> MHLSLLVPFLFWITGCCTAEDPVTGPEEVSGQEQGSLTVQCRYTSGWKDYKKYWCQGVPQRSCKTLVETDASEQLVKKNRVSIRDNQRDFIFTVTMEDLRMSDAGIYWCGITKGGLDPMFKVTVNIGPVPTMPPITSTTTIFTVTTTVKETSMFPTLTSYYSDNGHGGGDSGGGEDGVGDGFLDLSVLLPVISAVLLLLLLVASLFAWRMVRRQKKAAGPPSEQAQSLEGDLCYADLSLKQPRTSPGSSWKKGSSMSSSGKDHQEEVEYVTMAPFPREEVSYAALTLAGLG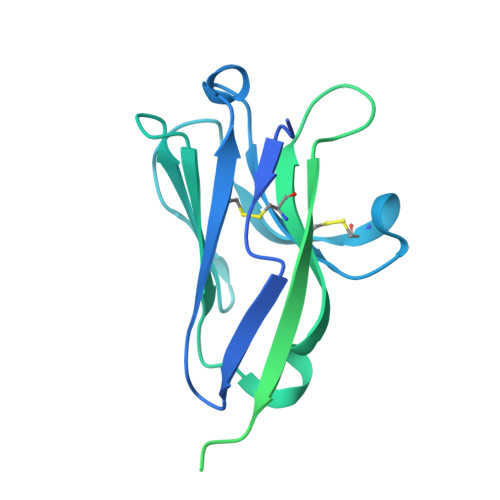QEPTYGNTGCPITHVPRTGLEEETTEYSSIRRPLPAAMP> MFIRIKCFSKQPI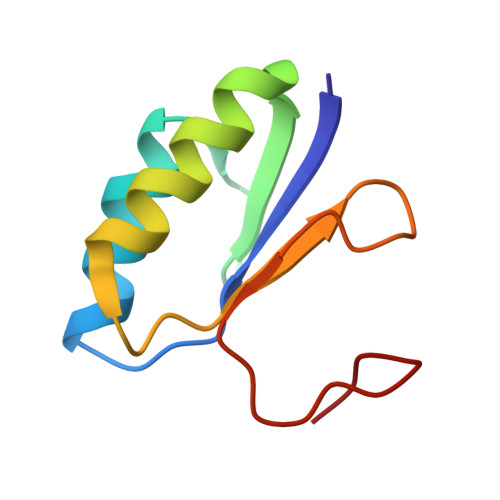AKKVSREVSAYLEYTGNNTWEGHISGQGVSNLQTKLINVGKGVKVVCNYQDKVLFAIGNVAMSDTGSV> NKALNLQC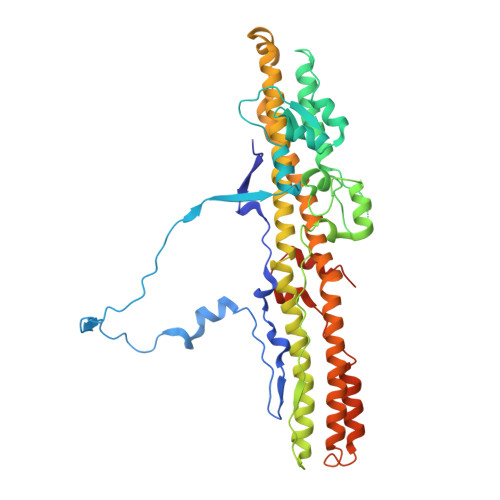IDVDNEDLFFIADKNSFSDDLSKNERIEYNTQSNYIENDFPINELILDTDLISKIELPSENTESLTDFNVDVPVYEKQPAIKKIFTDENTIFQYLYSQTFPLDIRDISLTSSFDDALLFSNKVYSFFSMDYIKTANKVVEAGLFAGWVKQIVNDFVIEANKSNTMDKIADISLIVPYIGLALNVGNETAKGNFENAFEIAGASILLEFIPELLIPVVGAFLLESYIDNKNKIIKTIDNALTKRNEKWSDMYGLIVAQWLSTVNTQFYTIKEGMYKALNYQAQALEEIIKYRYNIYSEKEKSNINIDFNDINSKLNEGINQAIDNINNFINGCSVSYLMKKMIPLAVEKLLDFDNTLKKNLLNYIDENKLYLIGSAEYEKSKVNKYLKTIMPFDLSIYTNDTILIEMFNKYNSLEALASGHHHHHH L-gamma-glutamyl-S-[(3R)-1-ethyl-2,5-dioxopyrrolidin-3-yl]-L-cysteinylglycine | C16 H24 N4 O8 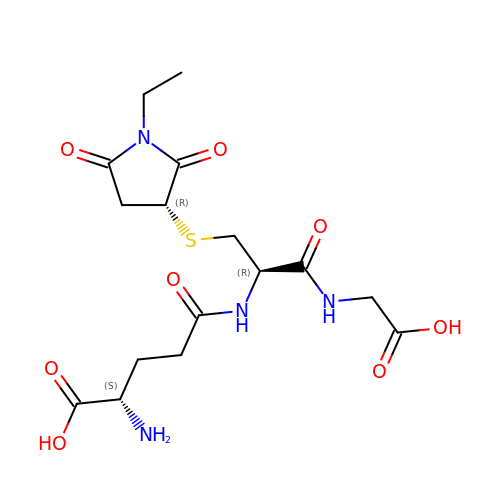S | QCPAUAAIPLHRLB-LPEHRKFASA-N>[2x]MAHHHHHHMAYFLEQTDSEIFELIFEEYKRQNEHLEMIASENYTFPSVMEAMGSILTNKYAEGYPNKRYYGGCEVVDKIESLAIERAKKLFNCQFANV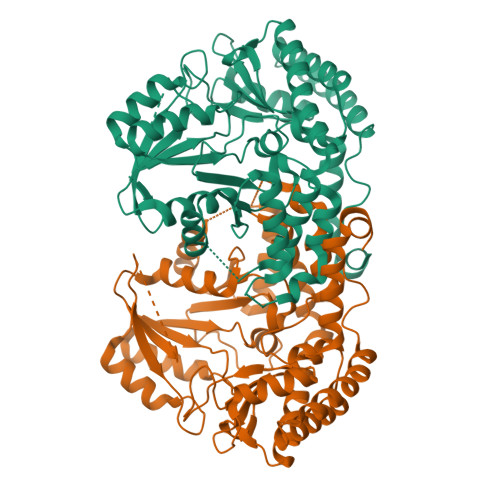QAHSGSQANNAVYHALLKPYDKILGMDLSCGGHLTHGAKVSLTGKHYQSFSYGVNLDGYIDYEEALKIAQSVKPEIIVCGFSAYPREIDFKKFREIADEVGALLLGDIAHVAGLVVTNEHAHPFPHCHVVSSTTHKTLRGPRGGIILTNDEEIAAKIDKAIFPGTQGGPLMHVIAAKAVGFKENLKPEFKAYAKLVKSNMQVLAKALKEKNHKLVSGGTSNHLLLMDFLDKPYSGKDADIALGNAGITVNKNTIPGETRSPFVTSGIRIGSAALSARGMGAKEFEIIGNKISDILNDINNVSLQLHVKEELKAMANQFPVYQQPIF>[2x]MNIHEWQSKQLIQKYGGRAQSGEVAFSPERSRDIAKKLWNQFPGCEFVVKAQVLAGGRGKG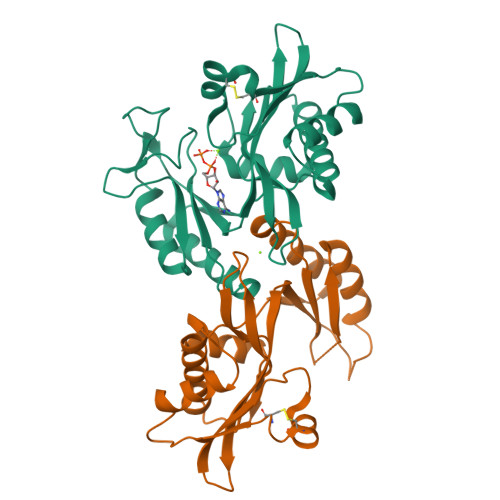HWEHGMQGGVKLAKTPEEVYEIANEMIGHKLITKQTGAKGINCNKVMVCGAVKILKEFYLSILLDRAMGCPVIIATSQGGMGIEEVAQKCPECLFKVPISVKNGPTNEQLVKLAKDLGLEGDLVQDCVDNVKALYQVFDKCDSTMVEINPLGVIETPTDEKVICCLDAKIAFDKDAAFGLEHHHHHHHH>LTAKHRPSVVWLHNAECTGCTEAAIRTIKPYIDALILDTISLDYQETIMAAAGEAAEAALHQALEGKDGYYLVVEGGLPTIDGGQWGMVAGHPMIETTKKAAAKAKGIICIGTCSAYGGVQKAKPNPSQAKGVSEALGVKTINIPGCPPNPINFVGAVVHVLTKGIPDLDENGRPKLFYGELVHDNCPRLPHFEASEFAPSFDSEEAKKGFCLYELGCKGPVTYNNCPKVLFNQVNWPVQAGHPCLGCSEPDFWDTMTPFYEQG[3x];>[3x]MAESKPTPQSTFTGPIVVDPITRIEGHLRIMVEVENGKVKDAWSSSQLFRGLEIILKGRDPRDAQHFTQRACGMCTYVHALASSRCVDDAVKVSIPANARMMRNLVMASQYLHDHLVHFYHMHALDWVDVTAALKADPNKAAKLAASIAPARPGNSAKALKAVQDKLKAFVESGQLGIFTNAYFLGGHKAYYLPPEVDLIATAHYLEALHMQVKAASAMAILGGKNPHTQFTVVGGCSNYQGLTKDPLANYLALSKEVCQFVNECYIPDLLAVAGFYKDWGGIGGTSNYLAFGEFATDDSSPEKHLATSQFPSGVITGRDLGKVDNVDLGAIYEDVKYSWYAPGGDGKHPYDGVTDPKYTKLDDKDHYSWMKAPRYKGKAMEVGPLARTFIAYAKGQPDFKKVVDMVLGKLSVPATALHSTLGRTAARGIETAIVCANMEKWIKEMADSGAKDNTLCAKWEMPEESKGVGLADAPRGALSHW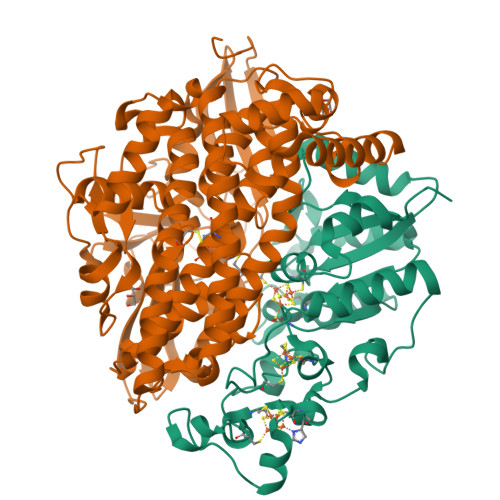IRIKGKKIDNFQLVVPSTWNLGPRGAQGDKSPVEEALIGTPIADPKRPVEILRTVHAFDPCIACGVH>[2x]MNYPAEPFRIKSVETVSMIPRDERLKKMQEAGYNTFLLNSKDIYIDLLTDSGTNAMSDKQWAGMMMGDEAYAGSENFYHLERTVQELFGFKHIVPTHQGRGAENLLSQLAIKPGQYVA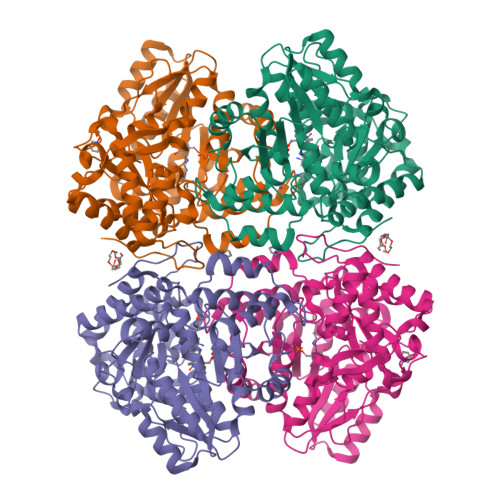GNMYFTTTRYHQEKNGAVFVDIVRDEAHDAGLNIAFKGDIDLKKLQKLIDEKGAENIAYICLAVTVNLAGGQPVSMANMRAVRELTEAHGIKVFYDATRCVENAYFIKEQEQGFENKSIAEIVHEMFSYADGCTMSGKKDCLVNIGGFLCMNDDEMFSSAKELVVVYEGMPSYGGLAGRDMEAMAIGLREAMQYEYIEHRVKQVRYLGDKLKAAGVPIVEPVGGHAVFLDARRFCEHLTQDEFPAQSLAASIYVETGVRSMERGIISAGRNNVTGEHHRPKLETVRLTIPRRVYTYAHMDVVADGIIKLYQHKEDIRGLKFIYEPKQLRFFTARFDYI>MEIVEYPDPILRAKNKRIDIFDENLKNLVDAMFDVMYKTDMIGLSAPQVGLNVQLMVFNPAGEPGEGKEIVLVNPKIKKYSDKLVPFDEGCLSFPGIYAEVVRPQSVKIDARDITGERFSISLSRLPARIFQHEYDHLEGVLFFDRMTDQVLDSIREELEALEKKYEEKTGLPSPERVEARQKRKAGVGFGKR[2x]

Here, we explore the precise structural inhibitory mechanism of actinonin, which is a slow, tight-binding inhibitor of peptide deformylase (PDF), a metal cation-dependent enzyme. PDF is the first enzyme in the N-terminal methionine excision pathway, an essential and ubiquitous process that contributes to the diversity of N-terminal amino acids. The function of the active-site metal is to activate the reactive water molecule involved in peptide hydrolysis. Actinonin is a natural product with antibiotic activity that inhibits PDF by mimicking the structure of its natural substrates (nascent peptide chains starting with Fo-Met-Aaa, where Fo is a formyl group and Aaa is any amino acid) in their transition state.

In this respect, site-directed mutagenesis of AtPDF was performed on Gly41, Ile42, and Ile130. The two most interesting variants, G41Q and G41M, could be crystallized under the same conditions as the WT protein. In contrast, the 3D structure of the G41M variant showed that the asymmetric unit was composed of two molecules with distinct structures. One molecule (chain A) is in the O state and is similar to the structures of the WT and the G41Q variant (zone “O”). Ringer analysis indicates that in the free G41M variant, many residues show evidence for unmodeled alternate conformers—including positions 58, 42, and 130—in keeping with the second hypothesis. A very similar situation—although more balanced between the two states—appears to occur in the case of variant G41M, suggesting that a mechanism involving conformational selection followed by induced fit is a general model for PDF and that AtPDF is a specific case where population shift virtually does not occur as the free enzyme is completely in the O conformation. In support of this hypothesis, recent data show that the 3D structure of a C-terminally truncated, poorly active version of AtPDF is in the C conformation in the unbound state, although crystallized under conditions identical to ours. This structure is similar to that of chain B, one of the two molecules of the asymmetric subunit of variant G41M.> MTTTERPDLAWLDEVTMTQLERNPYEVYERLRAEAPLAFVPVLGSYVASTAEVCREVATSPDFEAVITPAGGRTFGHPAIIGVNGDIHADLRSMVEPALQPAEVDRWIDDLVRPIARRYLERFENDGHAELVAQYCEPVSVRSLGDLLGLQEVDSDKLREWFAKLNRSHTNAAVDENGEFANPEGFAEGDQAKAEIRAVVDPLIDKWIEHPDDSAI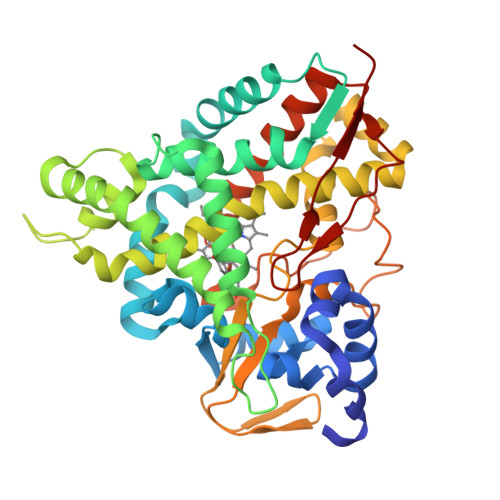SHWLHDGMPPGQTRDREYIYPTIYVYLLGAMQEPGHGMASTLVGLFSRPEQLEEVVDDPTLIPRAIAEGLRWTSPIWSATARISTKPVTIAGVDLPAGTPVMLSYGSANHDTGKYEAPSQYDLHRPPLPHLAFGAGNHACAGIYFANHVMRIALEELFEAIPNLERDTREGVEFWGWGFRGPTSLHVTWEV>MDTFVLDTSVFTNPDVYHQFEEDQLGAIENFISLASHTNANFFMPTSVYYEFTKMVSLGDLAPKFELVVRIRSPRKWGLMVPAEFLYEFIEEVRYRINKGLRIAEEHTKEAGKLAEEEVGRVVNRLREKYREALRAGIIDSKEDVDVLLLSYELDAILVSGDEGLRKWADRVGIKLIDPKNLRYIMENLTKVGR[7x]

One of the first steps of tRNA processing in nearly every organism is the removal of the 5′ leader sequence by ribonuclease P (RNase P). In contrast to other RNase Ps, HARPs consist only of a metallonuclease domain and lack the canonical substrate recognition domain essential in other classes of proteinaceous RNase P. We determined the cryo-EM structure of Aquifex aeolicus HARP (Aq880) and two crystal structures of Hydrogenobacter thermophilus HARP (Hth1307) to reveal that both enzymes form large ring-like assemblies: a dodecamer in Aq880 and a tetradecamer in Hth1307. HARP structures in additional oligomeric states have also been published, including HARP dimers from Planctomyces bacterium and Thermococcus celer and a HARP tetramer from P. bacterium complexed with Escherichia coli pre-tRNAHis. These data all show that a monomer of HARP is a VapC-like endonuclease that consists of a PIN domain-like metallonuclease domain and two protruding α helices, which are thought to be responsible for substrate recognition. The active site is conserved among HARPs and PRORPs, with five negatively charged residues, predominantly aspartate, positioned to coordinate two catalytic magnesium ions.

Molecular replacement revealed a heptamer in the asymmetric unit that, upon generation of its symmetry mate, produces a tetradecamer (14-mer) flat cylindrical ring consisting of a radial arrangement of seven HARP dimers. The structure was solved to 3.2 Å resolution. Notably, the dimer and tetramer interfaces of the 14-mer are fairly similar when compared to our Hth1307 tetramer structure. The angles between dimers in the 14-mer structure range from 48° to 54°, and the distances between the proposed tRNA elbow binding region and the active site ranges from 39.4 to 42.1 Å. Despite the additional dimer compared to the dodecamers, the Hth1307 tetradecamer maintains a roughly 42 Å distance from the active site to the proposed binding site. The tetradecamer presented here is the largest oligomeric HARP assembly to be described so far. Strikingly, unlike all of the dodecameric structures, our tetradecameric structure has no helical features and is instead a flat ring with nearly identical tetramer interfaces throughout. Experiments using His-tagged Hth1307 revealed a single oligomeric state of a tetradecamer (14-mer). The ability of Hth1307 to form a 14-mer in vitro was confirmed using native MS experiments, providing evidence that a 14-mer structure is not an artifact of our crystallization conditions.> MFLPPPECPVFEPSWEEFADPFAFIHKIRPIAEQTGICKVRPPPDWQPPFACDVDKLHFTPRIQRLNELEAQTRVKLGGGGARDYTLRTFGEMADAFKSDYFNMPVHMVPTELVEKEFWRLVSTIEEDVTVEYGADIASKEFGSGFPVRDGKIKLSPEEEEYLDSGWNLNNMPVMEQSVLAHITADICGMKLPWLYVGMCFSSFCWHIEDHWSYSINYLHWGEPKTWYGVPGYAAEQLENV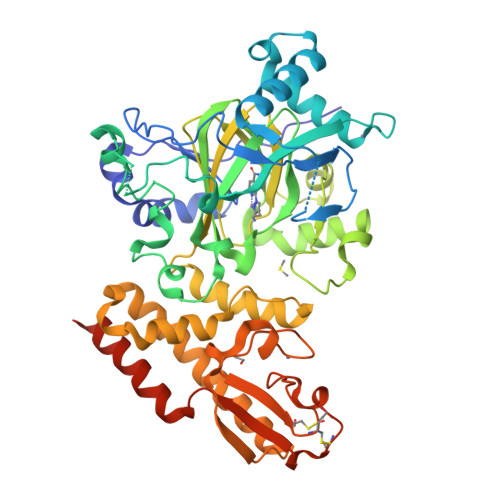MKKLAPKLFVSQPDLLHQLVTIMNPNTLMTHEVPVYRTNQCAGEFVITFPRAYHSGFNQGFNFAEAVNFCTVDWLPLGRQCVEHYRLLHRYCVFSHDEMICKMASKADVLDVVVASTVQKDMAIMIEDEKALRETVRKLGVIDSERMDFELLPDDERQCVKCKTTCFMSAISCSCKPGLLVCLHHVKELCSCPPYKYKLRYRYTLDDLYPMMNALKLRAESYNEWALNVNEALEAKINK> GSDSRTVSELVTNTNTIRVAMKDAYQRDGKYPDYQAPLSLTADSIKTDSTGIAVAQLVQLGKLTPDEARNGISGDYIGIGGAITSSGSTINKGFAMELNGLSQEQCRSILGQVGDNWEYVAVGTSPSGSYDALSAGAVNMLAATDNTTILRSLAANGQVSLTAEKILK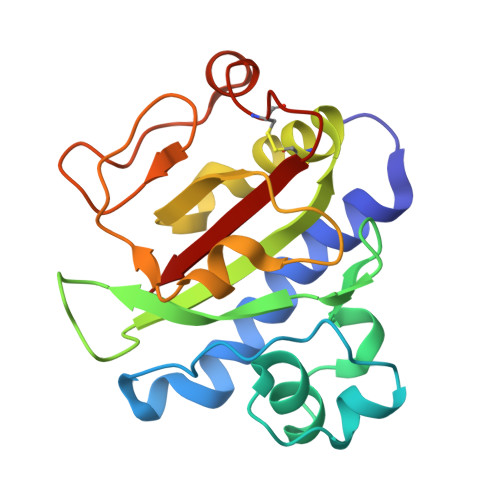TCTATVNSITLASR> FVPNVHAAEFVPS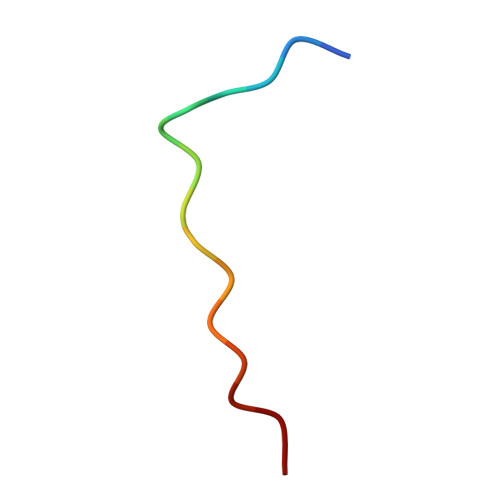FL>MSRRPWLLALALAVALAAGSAGASTGSDATVPVATQDGPDYVFHRAHERMLFQTSYTLENNGSVICIPNNGQCFCLAWLHSRGTPGEKIGAQVCQWIAFSIAIALLTFYGFSAWKATCGWEEVYVCCVEVLFVTLEIFKEFSSPATVYLSTGNHAYCLRYFEWLLSCPVILIKLSNLSGLKNDYSKRTMGLIVSCVGMIVFGMAAGLATDWLKWLLYIVSCIYG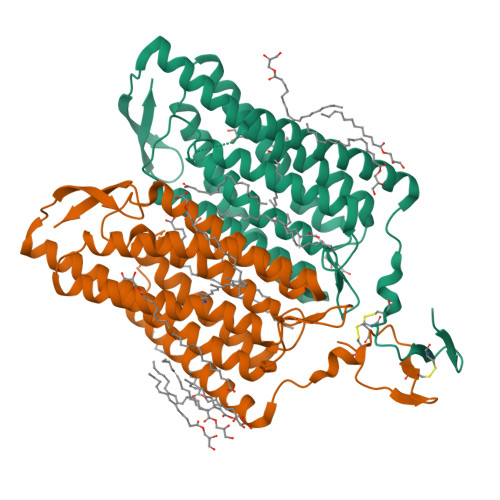GYMYFQAAKCYVEANHSVPKGHCRMVVKLMAYAYFASWGSYPILWAVGPEGLLKLSPYANSIGHSICDIIAKEFWTFLAHHLRIKIHEHILIHGDIRKTTKMEIGGEEVEVEEFVEEEDEDTV[2x]> MGTVSSRRSWWPLPLLLLLLLLLGPAGARAQEDEDGDYEELVLALRSEEDGLAEAPEHGTTATFHRCAKDPWRLPGTYVVVLKEETHLSQSERTARRLQAQAARRGYLTKILHVFHGLLPGFLVKMSGDLLELALKLPHVDYIEEDSSVFAQSIPWNLERITPPRYSADEYQPPDGGSLVEVYLLDTSIQSDHREIEGRVMVTDFENVPEEDGTRFHRQASKCDSHGTHLAGVVSGRDAGVAKGASMRSLRVLNCQGKGTVSGTLIGLEFIRKSQLVQPVGPLVVLLPLAGGYSRVLNAACQRLARAGVVLVTAAGNFRDDACLYSPASAPEVITVGATNAQDQPVTLGTLGTNFGRCVDLFAPGEDIIGAS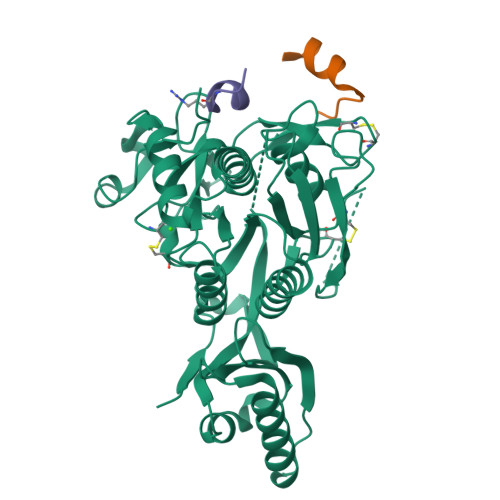SDCSTCFVSQSGTSQAAAHVAGIAAMMLSAEPELTLAELRQRLIHFSAKDVINEAWFPEDQRVLTPNLVAALPPSTHGAGNSHHHHHH;> XTVFTSWEEYLDWVX;> XWNLVRIGLLR>[6x]SNASISMANPIKTYHLSNLTQTELLSLKSRPRIDFSSVFDIVNPIVDDVHAHGDAAVKQYTSKFDKVDLENIVELVSDLPDPVLDPAIKEAFDVAYSNIYAFHAAQKSPEKSVENMKGVQCKRVARSINSVGLYVPGGTAVLPSTALMLAVPAQIAGCKTIVLANPPTRDGTTCKEVLYCAKKAGVTHLLKAGGAQAISAMAWGTETCPKVEKIFGPGNQYVTAAKMILQNSEAMVSIDMPAGPSEVLVIADKHAIPSHVAADLLSQAEHGPDSQVVLVIAGDGVDQNAIQEEVSKQCQSLPRGEFAAKALSHSFIVHARDMLEAITFSNMYAPEHLIINVKDAEKWESFIENAGSVFLGSWTPESVGDYASGTNHVLPTYGYARMYSGVSLDSFLKYITVQSLTEEGLRKLGPYVETMAEVEGLEAHKRAVTLRLQDIEARQVSR

HDH (EC 1.1.1.23) is a bifunctional enzyme that oxidises L-histidinol (HOL) via L-histidinaldehyde (HAL) into His in two sequential reactions, each coupled with a reduction of one nicotinamide adenine dinucleotide (NAD+) molecule to NADH. We show three crystal structures of Zn2+-bound MtHDH complexed with: (i) imidazole (IMD); (ii) HOL; and (iii) His with NAD+. The three structures reported herein are isomorphous, with three dimers (AB, CD, and EF) forming the asymmetric unit. The MtHDH monomer is composed of four domains.

HOL coordinates Zn2+ with N and Nδ atoms. More precisely, the N atom occupies the same position as Wat1 in the MtHDH/IMD complex, whereas the imidazole moiety of HOL is bound in a manner similar to IMD. Like IMD, HOL also forms an H-bond with Glu455*. The O atom of HOL interacts with carbonyl O of His408 and Nε of His368. Upon HOL binding, a significant change takes place in the coordination sphere of Zn2+. The Oε of Gln299 substitutes Wat2, meaning that, in the HOL complex, the metal is coordinated only by the protein and the substrate atoms. One important change is a different conformation of Gln299. In the complex with HOL, where Gln299 no longer binds Ser277, the latter has an altered conformation. Although Gln299 belongs to domain II, this domain shows few conformational changes, whereas the majority of the rearrangements concern domain I. The most prominent movement involves a loop region from Pro273 to Ser277. Other conformational changes involve loop Pro168-Val173 and the loop with the N-terminal side of helix α10, Gly248-Tyr253. Rearrangement of the latter region flips the ψ angle of Pro249 by almost 155°, from −53.8° in the MtHDH/IMD complex to 151.3° in HOL complex.>KFPRVKNWEVGSITYDTLSAQAQQDGPCTPRRCLGSLVFPRKLQGRPSPGPPAPEQLLSQARDFINQYYSSIKRSGSQAHEQRLQEVEAEVAATGTYQLRESELVFGAKQAWRNAPRCVGRIQWGKLQVFDARDCRSAQEMFTYICNHIKYATNRGNLRSAITVFPQRCPGRGDFRIWNSQLVRYAGYRQQDGSVRGDPANVEITELCIQHGWTPGNGRFDVLPLLLQAPDEPPELFLLPPELVLEVPLEHPTLEWFAALGLRWYALPAVSNMLLEIGGLEFPAAPFSGWYMSTEIGTRNLCDPHRYNIL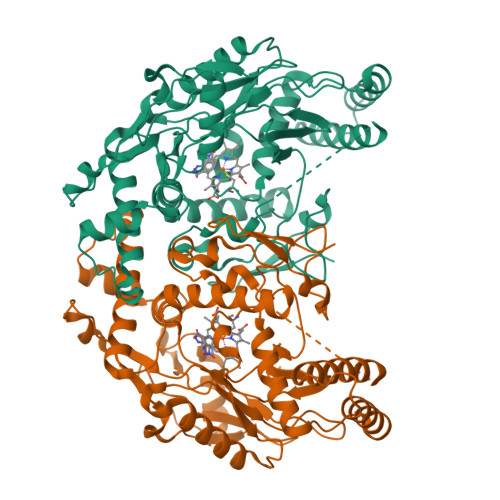EDVAVCMDLDTRTTSSLWKDKAAVEINVAVLHSYQLAKVTIVDHHAATASFMKHLENEQKARGGCPADWAWIVPPISGSLTPVFHQEMVNYFLSPAFRYQPDPWK[2x]> LNTNQSVSARNQNARVRTRRAVAANDTEAPQVKSGDYVVYRGESFEYYAEITDNSGQVNRVVIRNVEGGANSTYLSPNWVKYSTENLGRPGNATVQNPLRTRIFGEVPLNEIVNEKSYYTRYIVAWDPSGNATQMVDNANRNGLERFVLTVKSQNEKYDPAESSVTYVNNLSNLSTSEREAVAAAVRAANPNIPPTAKITVSQNGTVTITYPDKSTDTIPANRVVKDLQISKSN

Many streptococci adhere to protein-attached carbohydrates expressed on cell surfaces using Siglec-like binding regions (SLBRs). Siglec-like binding regions (SLBRs) are among the streptococcal adhesive modules that bind sialoglycans. SLBRs contain two adjacent modules: a Siglec domain, which shares some features with mammalian Siglecs, and a Unique domain13 with no close homologs outside of the family. The conserved sialic acid-recognition motif governs general specificity while sequence diversity in surrounding loop regions allows the SLBR to select between related sialoglycans.

For SLBRHsa, this included structures from crystals soaked with the high-affinity ligands sTa and sLeC, the intermediate-affinity ligand 3’sLn, and the low-affinity ligand 6S-sLeX. The resolution ranged from 1.3 Å to 2.4 Å and the diffraction quality loosely correlated with ligand affinity. Instead, comparing costructure determined with sTa with the costructure determined with sLeC shows that the position of the EF loop differs by 5.9 Å. In the strong and intermediate ligands, the invariant Neu5Acα2-3 Gal effectively superimposes and has similar hydrogen bonds. Differences in the SLBR-ligand interactions predominantly map to the variable third sugar of the glycan. Biding strength may therefore be related to these interactions.> MGSQVSTQRSGSHENSNSATEGSTINYTTINYYKDSYAATAGKQSLKQDPDKFANPVKDIFTEMAAPLKSPSAEACGYSDRVAQLTIGNSTITTQEAANIIVGYGEWPSYCSDSDATAVDKPTRPDVSVNRFYTLDTKLWEKSSKGWYW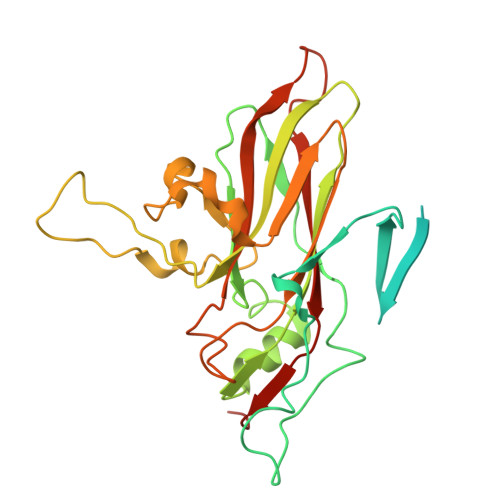KFPDVLTETGVFGQNAQFHYLYRSGFCIHVQCNASKFHQGALLVAVLPEYVIGTVAGGTGTEDSHPPYKQTQPGADGFELQHPYVLDAGIPISQLTVCPHQWINLRTNNCATIIVPYINALPFDSALNHCNFGLLVVPISPLDYDQGATPVIPITITLAPMCSEFAGLRQAVTQ>[2x]MAPDPKLPSADLPSQKQVIELLDGEFARAGYEIDDVVVNAATRPARITIVADGDKGLDLDAVAMLSRLASGLLDTVDTGDTPYVLEVTSP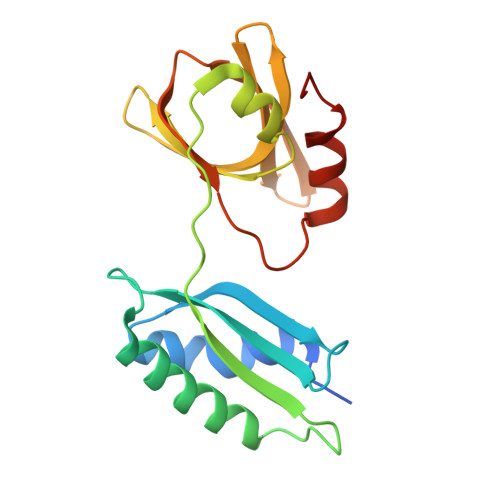GVDRPLTTEKHFRRARGRKAELSLADGSSLTARLGGTDGDQVNVVVAQGKDFAVRQIPLREITKAVVQVEFSPPNRRELELAEQTGKGARA> RLIHVSRCEMGTSTHRCWPRPCDTSSDEPISFWP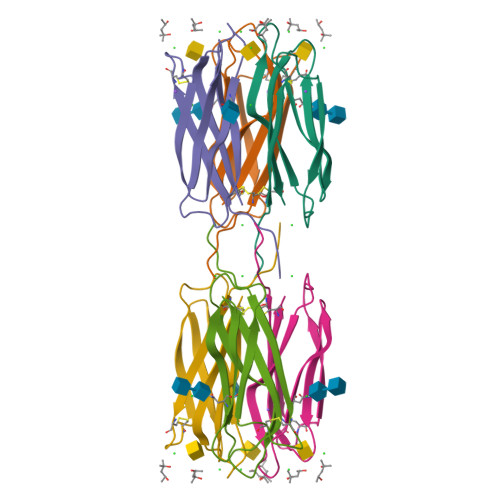PFENTPNVIVSFGMLDVDNSNNLRVNSSADDVTVGGFTLHYNSWYTTTVWNYKLIWIACD> MGSSHHHHHHSSGRENLYFQGVPMNIKGLFEVAVKVKNLEKSSQFYTEILGFEAGLLDSARRWNFLWVSGRAGMVVLQEEKENWQQQHFSFRVEKSEIEPLKKALESKGVSVHG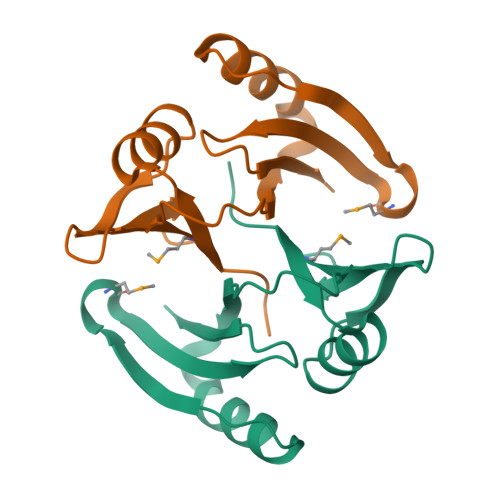PVNQEWMQAVSLYFADPNGHALEFTAL>XEWEALEKKLAALESKL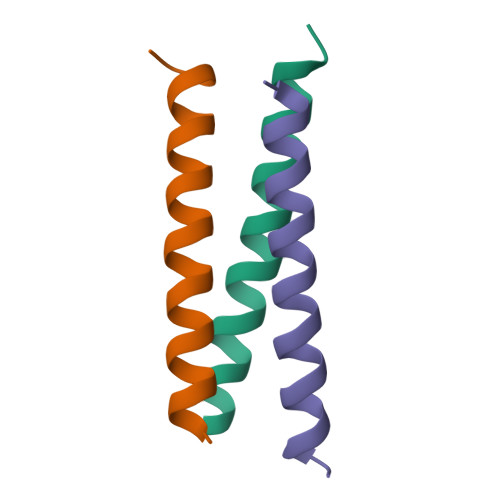QALEKKLEALEHGX[3x]>[2x]SMALQADFDRAAEDVRKLKARPDDGELKELYGLYK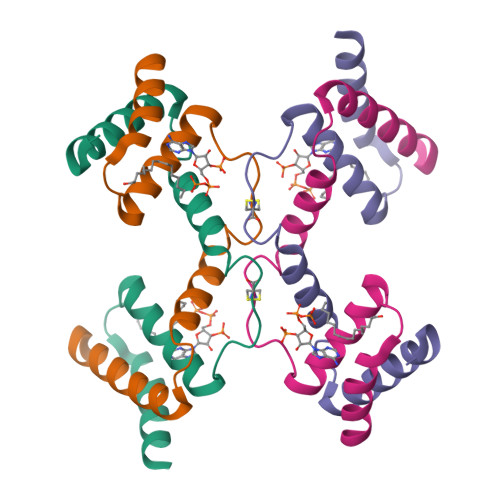QAIVGDINIACPGMLDLKGKAKWEAWNLKKGLSTEDATSAYISKAKELIEKYGI> SGVIKPDMKIKLKMEGNVNGYAFVIEGEGEGKPYDGTNTINLEVKEGAPLPFSYDILTTAFAYGNRAFTKYPDDIPNYFKQSFPEGYSWERTMTFEDK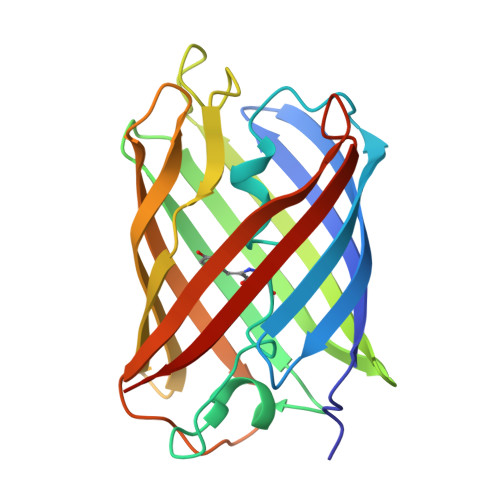GIVKVKSDISLEEDSFIYEIYLKGENFPPNGPVMQKKTTGWDASTERMYVRDGVLKGDVKHKLLLEGGGYYRVDFKTIYRAKKAVKLPDYHFVDHRIEELNHDKDHNKVTVYESAVARNSTD> MEDKGKTFFGQPLGLSTLFMTEMWERFSYYGMRAILLYYMWFLISTGDLHITRATAASIMAIYASMVYLSGTIGGFVADRIIGARPAVFWGGVLIMLGHIVLALPFGASALFGSIILIIIGTGFLKPNVSTLVGTLYDEHDRRRDAGFSIFVFGINLGAFIAPLIVGAAQEAAGYHVAFSLAAIGMFIGLLVYYFGGKKTLDPHYLRPTDPLAPEEVKPLLVKVSLAVAGFIAIIVVMN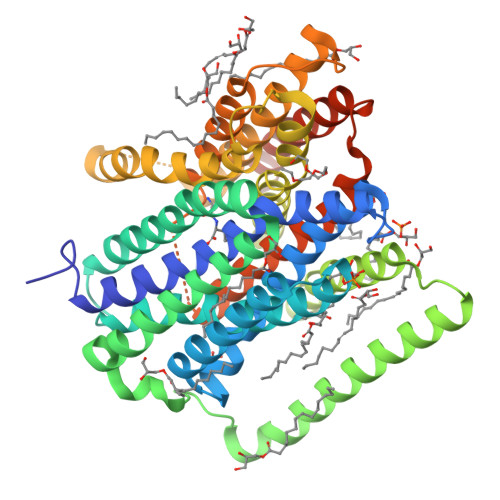LVGWNSLPAYINLLTIVAIAIPVFYFAWMISSVKVTSTEHLRVVSYIPLFIAAVLFWAIEEQGSVVLATFAAERVDSSWFPVSWFQSLNPLFIMLYTPFFAWLWTAWKKNQPSSPTKFAVGLMFAGLSFLLMAIPGALYGTSGKVSPLWLVGSWALVILGEMLISPVGLSVTTKLAPKAFNSQMMSMWFLSSSVGSALNAQLVTLYNAKSEVAYFSYFGLGSVVLGIVLVFLSKRIQGLMQGVEAENLYFQ> 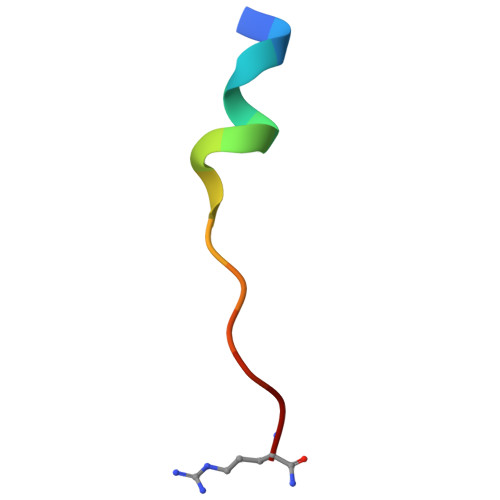AEGEFYKLKIRTPR Yellow fever virus (YFV) is a re-emerging flavivirus that causes severe hepatic disease and mortality in humans. Crystallographic studies have resolved the structure of the YFV E protein and shown that its domain architecture is similar to related flaviviruses, with three N-terminal ectodomains, known as domains I (DI), II (DII) and III (DIII) and a stem anchor region known as the transmembrane domain (TM). Here we use a chimeric virus platform to resolve the first high resolution cryo-EM structures of YFV. Stark differences in particle morphology and homogeneity are observed between vaccine and virulent strains of YFV, and these are found to have significant implications on antibody recognition and neutralisation.

Given that DIII of 17D was critical in improving the particle homogeneity of bYFVES504, we next examined whether swapping DIII between bYFV17D and bYFVAsibi would have a similar effect. Remarkably, the bYFV17D/DIIIAsibi particles most closely resembled the phenotype of the virulent bYFVs, whilst the bYFVAsibi/DIII17D particles most closely resembled the phenotype of bYFV17D. We then resolved the 3D structure of bYFVAsibi/DIII17D to a resolution of 5.5 Å. The symmetry expansion method was also used to further refine the ASU of bYFVAsibi/DIII17D to 3.6 Å. Similar to previous ASU maps, the bYFVAsibi/DIII17D ASU map shows lower local resolution at the icosahedral three-fold axis, as well as no clear TM domains for M or E. This cryo-EM map was then used to build an atomic model of the bYFVAsibi/DIII17D ASU, which was found to be highly similar to the bYFVES504/DIII17D ASU model with a Cα RMSD of 0.85 Å. Furthermore, incorporation of YFV17D DIII into bYFVAsibi also switched virion homogeneity and FLE mAb neutralisation sensitivity phenotypes.

>AHCIGITDRDFIEGVHGGTWVSATLEQDKCVTVMAPDKPSLDISLETVAIDGPAEARKVCYNAVLTHVKINDKCPSTGEAHLAEENEGDNACKRTYSDRGWGNGCGLFGKGSIVACAKFTCAKSMSLFEVDQTKIQYVIRAQLHVGAKQENWNTDIKTLKFDALSGSQEAEFTGYGKATLECQVQTAVDFGNSYIAEMEKESWIVDRQWAQDLTLPWQSGSGGVWREMHHLVEFEPPHAATIRVLALGNQEGSLKTALTGAMRVTKDTNDNNLYKLHGGHVSCRVKLSALTLKGTSYKICTDKMFFVKNPTDTGHGTVVMQVKVSKGAPCRIPVIVADDLTAAINKGILVTVNPIASTNDDEVLIEVNPPFGDSYIIVGRGDSRLTYQWHK[3x]N-(thiophen-2-yl)acetamide | C6 H7 N O S | 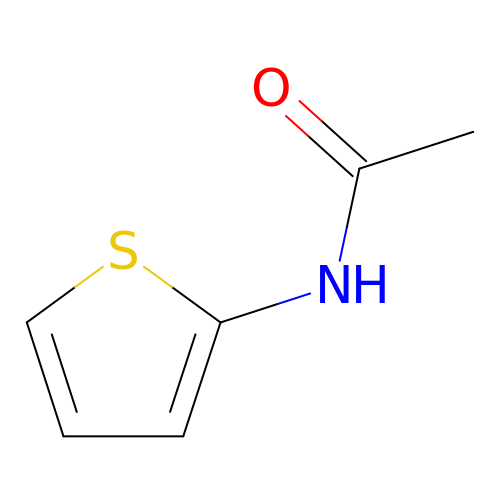FSATURPVOMZWBY-UHFFFAOYSA-N6-[2-(phenoxymethyl)-1,3-thiazol-4-yl]-3,4-dihydro-1H-quinolin-2-one | C19 H16 N2 O2 S | 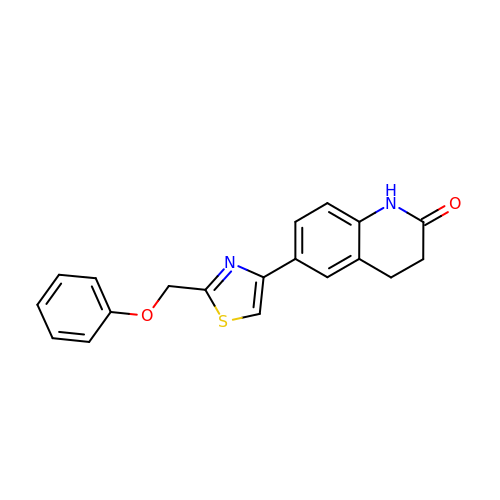QXHYTMRDSBLWLI-UHFFFAOYSA-N> GSHMRPSMKLVKFRKGDSVGLRLAGGNDVGIFVAGVLEDSPAAKEGLEEGDQILRVNNVDF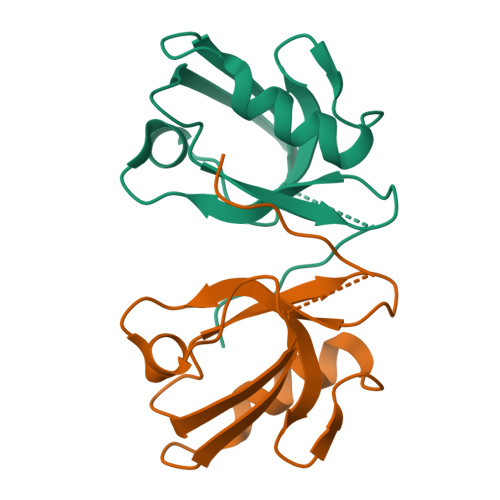TNIIREEAVLFLLDLPKGEEVTILAQKKKAAGGGLWFSDWL Bacteriophage Casadabanvirus JBD30, from the order Caudoviricetes, is a temperate phage that infects the bacterium Pseudomonas aeruginosa. The virion of bacteriophage JBD30 is composed of an icosahedral capsid, long flexible non-contractile tail, and a baseplate. Using its baseplate, JBD30 attaches to Pseudomonas aeruginosa via the bacterial type IV pilus, whose subsequent retraction brings the phage to the bacterial cell surface.

The JBD30 portal protein (gp32) has the same domain organization as portals of other dsDNA phages, such as T4, SPP1, and T7. It is composed of crown, wing, stem, and clip domains. The diameter of the portal channel at its narrowest is 30 Å in a virion and 21 Å in an empty JBD30 particle. The difference is caused by the conformational change of helices α12 from the wing domains and tunnel loops of the portal proteins.

> MAQIVDVYGNPIRTQQLREPQTSRLAGLAKEFAQHPAKGLTPAKLARILVEAEQGNLQAQAELFMDMEERDAHLFAEMSKRKRAILGLDWAVEPPRNASAAEKADADYLHELLLDLEGLEDLLLDALDGIGHGYSCIELEWALQGREWMPLAFHHRPQSWFQLNPEDQNELRLRDNSPAGEALQPFGWIIHRPRARSGYVARSGLFRVLAWPYLFRHYATSDLAEMLEIYGLPIRLGKYPPGTADEEKATLLRAVTGLGHAAAGIIPETMAIDFQQAAQGSSDPFLAMMRQSEDAISKAVLGGTLTSTTSQSGGGAFALGQVHNEVRHDLLASDARQLAATLSRDLLWPLLVLNRPGSPDVRRAPRLVFDLREQADITSMAQSIPALVNVGLEIPSAWVYDKLGIPQPAKNEPVLRSAAQPAILSRQHGQRVAALATIVGPRYGDQQALDKALASLPAKDMQDQVNDLLAPLLEAVNRGDSETELLGALAEAFPDMDDSALTDALHRLLFAADTWGRLHGNLDRID;> MSYCTLADLIEQYSEQKIREVSDRVNKPATTIDTVIVDRAIADADSEIDLHLHGRYQLPLASVPTALKRIACGLAYANLHIVLKEENPVYKTAEHLRKLLSGIANGKLSLALDADGKPAPVANTVQISEGRNDWGADW>CTTTTAAAAG[2x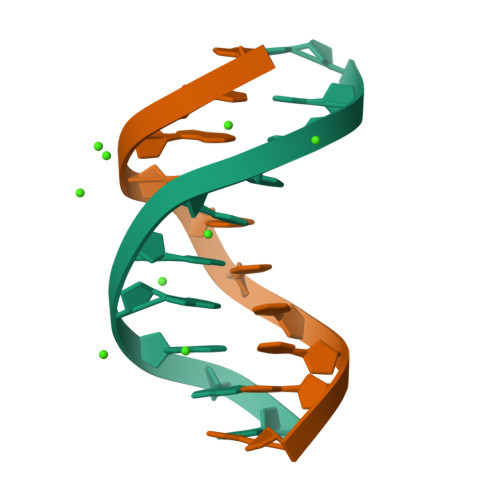]>MKSALVVSAHSADFVWRAGGAIALHAEQGYAMHVVCLSFGERGESAKLWRKGEMTEAKVKDARREEAMAAAEILGASVEFFDIGDYPMRADKDTLFRLADVYRRVQPEFVLSHSLKDPYNYDHPLAMHLAQEARIIAQAEGYKPGEKIVGAPPVYAFEPHQPEQCEWRPDTFLDITSVW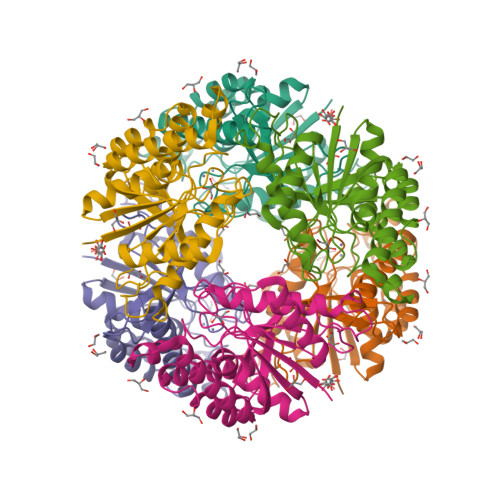DKKYAAIQCMAGQEHLWEYYTRVALQRGVQAKRNVGITSARNIVYAEGLQSVFPRVTENLA[2x]> SNAMAKTLKDLQGWEIITTDEQGNIIDGGQKRLRRRGAKTEHYLKRSSDGIKLGRGDSVVMHNEAAGTYSVYMIQELRLNTLNNVVELWALTYLRWFEVNPLAHYRQFNPDANILNRPLNYYNKLFSETANKNELYLTAELAELQLFNFIRVANVMDGSKWEVLKGNVDPERDFTVRYICEPTGEKFVDINIEDVKAYIKKVEPREAQEYLKDLTLPSKKKEIKRGPQKKDKATQTAQISDAETRATDITDNEDGNEDESSDYESPSDIDVSEDMDSGEISADELEEEEDEEEDEDEEEKEARHTNSPRKRGRKIKLGKDDIDASVQPPPKKRGRKPKDPSKPRQMLLISSCRANNTPVIRKFTKKNVARAKKKYTPFSKRFKSIAAIPDLTSLPEFYGNSSELMASRFENKLKTTQKHQIVETIFSKVKKQLNSSYVKEEILKSANFQDYLPARENEFASIYLSAYSAIESDSATTIYVAGTPGVGKTLTVREVVKELLSSSAQREIPDFLYVEINGLKMVKPTDCYETLWNKVSGERLTWAASMESLEFYFKRVPKNKKKTIVVLLDELDAMVTKSQDIMYNFFNWTTYENAKLIVIAVANTMDLPERQLGNKITSRIGFTRIMFTGYTHEELKNIIDLRLKGLNDSFFYVDTKTGNAILIDAAGNDTTVKQTLPEDVRKVRLRMSADAIEIASRKVASVSGDARRALKVCKRAAEIAEKHYMAKHGYGYDGKTVIEDENEEQIYDDEDKDLIESNKAKDDNDDDDDNDGVQTVHITHVMKALNETLNSHVITFMTRLSFTAKLFIYALLNLMKKNGSQEQELGDIVDEIKLLIEVNGSNKFVMEIAKTLFQQGSDNISEQLRIISWDFVLNQLLDAGILFKQTMKN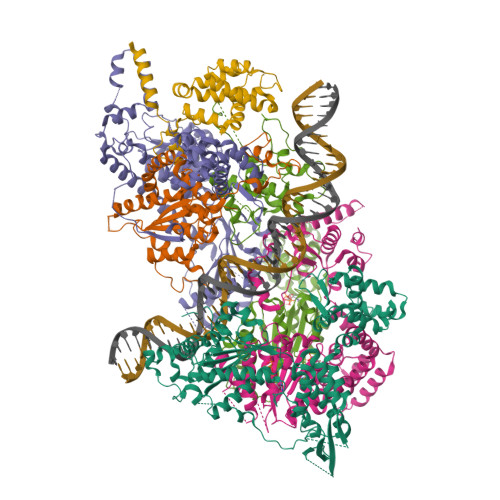DRICCVKLNISVEEAKRAMNEDETLRNL;> MLNGEDFVEHNDILSSPAKSRNVTPKRVDPHGERQLRRIHSSKKNLLERISLVGNERKNTSPDPALKPKTPSKAPRKRGRPRKIQEELTDRIKKDEKDTISSKKKRKLDKDTSGNVNEESKTSNNKQVMEKTGIKEKREREKIQVATTTYEDNVTPQTDDNFVSNSPEPPEPATPSKKSLTTNHDFTSPLKQIIMNNLKEYKDSTSPGKLTLSRNFTPTPVPKNKKLYQTSETKSASSFLDTFEGYFDQRKIVRTNAKSRHTMSMAPDVTREEFSLVSNFFNENFQKRPRQKLFEIQKKMFPQYWFELTQGFSLLFYGVGSKRNFLEEFAIDYLSPKIAYSQLAYENELQQNKPVNSIPCLILNGYNPSCNYRDVFKEITDLLVPAELTRSETKYWGNHVILQIQKMIDFYKNQPLDIKLILVVHNLDGPSIRKNTFQTMLSFLSVIRQIAIVASTDHIYAPLLWDNMKAQNYNFVFHDISNFEPSTVESTFQDVMKMGKSDTSSGAEGAKYVLQSLTVNSKKMYKLLIETQMQNMGNLSANTGPKRGTQRTGVELKLFNHLCAADFIASNEIALRSMLREFIEHKMANITKNNSGMEIIWVPYTYAELEKLLKTVLNTL;> MSDLNQSKKMNVSEFADAQRSHYTVYPSLPQSNKNDKHIPFVKLLSGKESEVNVEKRWELYHQLHSHFHDQVDHIIDNIEADLKAEISDLLYSETTQKRRCFNTIFLLGSDSTTKIELKDESSRYNVLIELTPKESPNVRMMLRRSMYKLYSAADAEEHPTIKYEDINDEDGDFTEQNNDVSYDLSLVENFKRLFGKDLAMVFNFKDVDSINFNTLDNFIILLKSAFKYDHVKISLIFNINTNLSNIEKNLRQSTIRLLKRNYHKLDVSSNKGFKYGNQIFQSFLDTVDGKLNLSDRFVEFILSKMANNTNHNLQLLTKMLDYSLMSYFFQNAFSVFIDPVNVDFLNDDYLKILSRCPTFMFFVEGLIKQHAPADEILSLLTNKNRGLEEFFVEFLVRENPINGHAKFVARFLEEELNITNFNLIELYHNLLIGKLDSYLDRWSACKEYKDRLHFEPIDTIFQELFTLDNRSGLLTQSIFPSYKSNIEDNLLSWEQVLPSLDKENYDTLSGDLDKIMAPVLGQLFKLYREANMTINIYDFYIAFRETLPKEEILNFIRKDPSNTKLLELAETPDAFDKVALILFMQAIFAFENMGLIKFQSTKSYDLVEKCVWRGI;> SNAMTISEARLSPQVNLLPIKRHSNEEVEETAAILKKRTIDNEKCKDSDPGFGSLQRRLLQQLYGTLPTDEKIIFTYLQDCQQEIDRIIKQSIIQKESHSVILVGPRQSYKTYLLDYELSLLQQSYKEQFITIRLNGFIHSEQTAINGIATQLEQQLQKIHGSEEKIDDTSLETISSGSLTEVFEKILLLLDSTTKTRNEDSGEVDRESITKITVVFIFDEIDTFAGPVRQTLLYNLFDMVEHSRVPVCIFGCTTKLNILEYLEKRVKSRFSQRVIYMPQIQNLDDMVDAVRNLLTVRSEISPWVSQWNETLEKELSDPRSNLNRHIRMNFETFRSLPTLKNSIIPLVATSKNFGSLCTAIKSCSFLDIYNKNQLSNNLTGRLQSLSDLELAILISAARVALRAKDGSFNFNLAYAEYEKMIKAINSRIPTVAPTTNVGTGQSTFSIDNTIKLWLKKDVKNVWENLVQLDFFTEKSAVGLRDNATAAFYASNYQFQGTMIPFDLRSYQMQIILQELRRIIPKSNMYYSWTQL;> MNVTTPEVAFREYQTNCLASYISADPDITPSNLILQGYSGTGKTYTLKKYFNANPNLHAVWLEPVELVSWKPLLQAIARTVQYKLKTLYPNIPTTDYDPLQVEEPFLLVKTLHNIFVQYESLQEKTCLFLILDGFDSLQDLDAALFNKYIKLNELLPKDSKINIKFIYTMLETSFLQRYSTHCIPTVMFPRYNVDEVSTILVMSRCGELMEDSCLRKRIIEEQITDCTDDQFQNVAANFIHLIVQAFHSYTGNDIFALNDLIDFKWPKYVSRITKENIFEPLALYKSAIKLFLSTDDNLSENGQGESAITTNRDDLENSQTYDLSIISKYLLIASYICSYLEPRYDASIFSRKTRIIQGRAAYGRRKKKEVNPRYLQPSLFAIERLLAIFQAIFPIQGKAESGSLSALREESLMKANIEVFQNLSELHTLKLIATTMNKNIDYLSPKVRWKVNVPWEIIKEISESVHFNISDYFSDIHE;> MSMQQVQHCVAEVLRLDPQEKPDWSSGYLKKLTNATSILYNTSLNKVMLKQDEEVARCHICAYIASQKMNEKHMPDLCYYIDSIPLEPKKAKHLMNLFRQSLSNSSPMKQFAWTPSPKKNKRSPVKNGGRFTSSDPKELRNQLFGTPTKVRKSQNNDSFVIPELPPMQTNESPSITRRKLAFEEDEDEDEEEPGNDGLSLKSHSNKSITGTRNVDSDEYENHESDPTSEEEPLGVQESRSGRTKQNKAVGKPQSELKTAKALRKRGRIPNSLLVKKYCKMTTEEIIRLCNDFELPREVAYKIVDEYNINASRLVCPWQLVCGLVLNCTFIVFNERRRKDPRIDHFIVSKMCSLMLTSKVDDVIECVKLVKELIIGEKWFRDLQIRYDDFDGIRYDEIIFRKLGSMLQTTNILVTDDQYNIWKKRIEMDLALTEPL>[5x]TVTYTNRVADARLGTFSQLLLQWKGSIYKLLYSEFLIFISLYFAISLVYRLILSESQRLMFEKLALYCNSYAELIPVSFVLGFYVSLVVSRWWAQYESIPWPDRIMNLVSCNVDGEDEYGRLLRRTLMRYSNLCSVLILRSVSTAVYKRFPSMEHVVRAGLMTPEEHKKFESLNSPHNKFWIPCVWFSNLAVKARNEGRIRDSVLLQGILNELNTLRSQCGRLYGYDWISIPLVYTQVVTVAVYSFFLACLIGRQFLDPEKAYPGHELDLFVPVFTFLQFFFYAGWLKVAEQLINPFGEDDDDFETNWLIDRNLQVSLMAVDEMHQDLPILEKDLYWNEPDPQPPYTAATAEYKRPSFLGSTFDISMQKEEMEFQPLEQIKENEEANHSTPLLGHLGRLLGVQSEGEEF

BEST1-4 proteins are expressed in the plasma membrane and form Ca2+-activated Cl- channels by assembling as pentamers. The channel comprises five BEST1 subunits arranged symmetrically around a central ion pore that is ~95 Å long. The diameter of the pore varies along its length and contains two constrictions, the ‘neck’ and the ‘aperture’, both of which are lined by hydrophobic amino acids. To address these questions we determined a series of cryo-electron microscopy (cryo-EM) structures of chicken BEST1 with and without Ca2+ in activated, deactivated, and inactivated states that represent the major gating transitions of the channel.

Inactivation is stimulated by high (>500 nM) concentrations of Ca2+ and is caused by the binding of a C-terminal ‘inactivation peptide’, contained within amino acids 346–367, to a receptor on the channel’s cytosolic surface that is located near the Ca2+ clasp. To begin studying the structural basis of gating in BEST1, we determined a 3.1 Å resolution cryo-EM structure of Ca2+-bound BEST1 without an antibody (the same construct used for X-ray studies, comprising residues 1–405 of chicken BEST1, and termed BEST1405). From single particle analysis we obtained only a single conformation, which indicates substantial conformational homogeneity among the ~300,000 channel molecules in the dataset. The conformation of the channel is indistinguishable from the previously published X-ray structure (Figure 1—figure supplements 1,2, RMSD for Cα atoms = 0.5 Å). As in the X-ray structure, each of the inactivation peptides, of which there are five owing to the symmetry of the channel, is bound to its cytosolic receptor and well defined in the density. Therefore, this cryo-EM structure also represents a Ca2+-bound inactivated state. This result indicates that antibody binding does not distort the channel from a native conformation and reflects a satisfying correspondence of structures determined using X-ray crystallography and cryo-EM methodologies. The channel inactivates at higher concentrations of Ca2+ through a mechanism that involves the binding of the C-terminal inactivation peptide to its receptor. The receptor is on the cytosolic surface of the channel and the binding of the inactivation peptide to it allosterically controls the conformation of the neck from a distance.> MLTL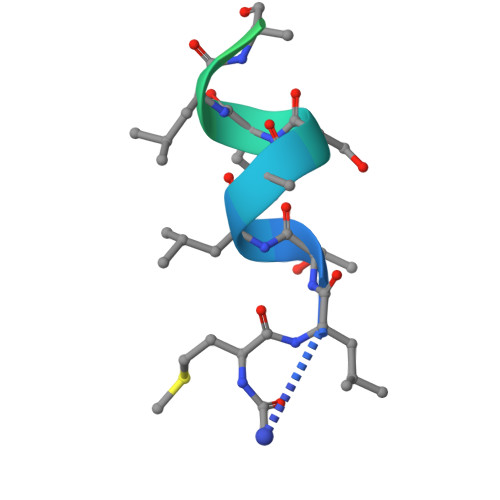ASKLKRDDGLKGSRTAATASD>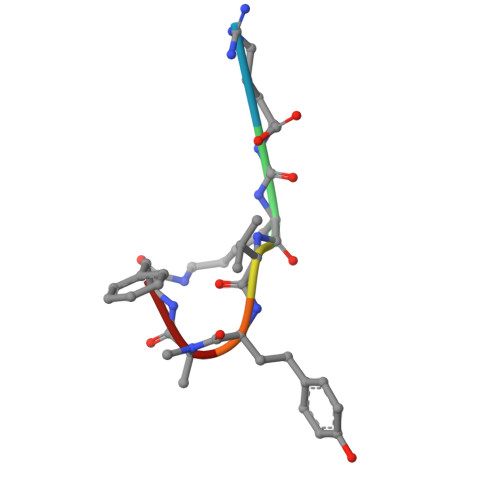 RKVYAF> GSASNPQTEEVSIKEIAITHHVKEGHEKADPSQFELLKVLGQGSFGKVFLVKKISGSDARQLYAMKVLKKATLKVRDRVRTKMERDILVEVNHPFIVKLHYAFQTEGKLYLILDFLRGGDLFTRLSKEVMFTEEDVKFYLAELALALDHLHSLGIIYRDLKPENILLDEEGHIKLTDFGLSKESIDHEKKAYSFCGTVEYMAPEVVNRRGHTQSADWWSFGVLMFEMLTGTLPFQGKDRKETMTM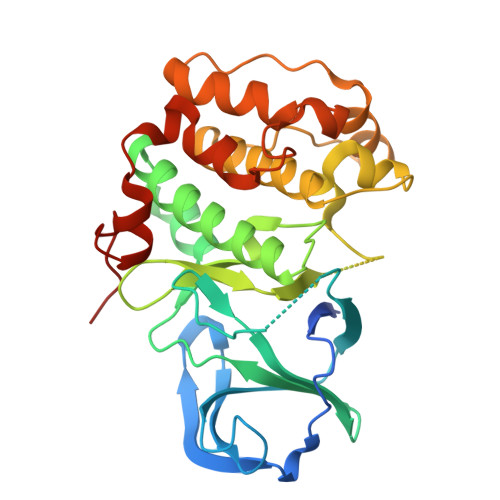ILKAKLGMPQFLSPEAQSLLRMLFKRNPANRLGAGPDGVEEIKRHSFFSTIDWNKLYRREIHPPFKPATGRP>MPLITTETGKKMHVLEDGRKLITVIPGDGIGPECVEATLKVLEAAKAPLAYEVREAGASVFRRGIASGVPQETIESIRKTRVVLKGPLETPVGYGEKSANVTLRKLFETYANVRPVREFPNVPTPYAGRGIDLVVVRENVEDLYAGIEHMQTPSVAQTLKLISWKGSEKIVRFAFELARAEGRKKVHCATKSNIMKLAEGTLKRAFEQVAQEYPDIEAVHIIVDNAAHQLVKRPEQFEVIVTTNMNGDILSDLTSGLIGGLGFAPSANIGNEVAIFEAVHGSAPKYAGKNVINPTAVLLSAVMMLRYLEEFATADLIENALLYTLEEGRVLTGDVVGYDRGAKTTEYTEAIIQNLGKTPRKTQVRGYKPFRLPQVDGAIAPIVPRSRRVVGVDVFVETNLLPEALGKALEDLAAGTPFRLKMISNRGTQVYPPTGGLTDLVDHYRCRFLYTGEGEAKDPEILDLVSRVA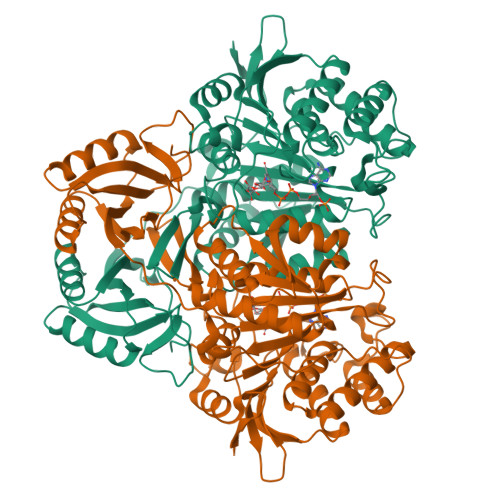SRFRWMHLEKLQEFDGEPGFTKAQGED[2x]During activation of a pentameric ligand-gated ion channel (pLGIC), the binding of agonists promotes the opening of a selective ion conduction pore at a distance of more than 50 Å away from the binding sites. Each subunit consists of a predominantly β-stranded extracellular domain and an α-helical transmembrane pore, which interact via an extended interface. Whereas ELIC forms a cation-selective channel with high conductance that is activated with high efficacy by the primary amines cysteamine, propylamine, and GABA, the cation-selective GLIC is activated by protons and inhibited by bulky positively charged compounds that also act as open channel blockers of the nAChR. Our study has identified a cluster of interacting residues located at the β1-β2 turn, the β6-β7 loop and the pre-M1 region of the extracellular domain, and the M2-M3 loop of the pore that exert a strong influence on channel function.

When mutating Thr28 in ELIC to aspartate, thereby introducing a negative charge that is present in many family members, the EC50 of channel activation shifts to a 45 times lower agonist concentration (18 μM). A similar increase in the affinity was observed in ITC experiments, where the agonist binds with a Keff of 90 μM, a 90-fold decrease in concentration compared to WT, while the binding of the antagonist acetylcholine was unchanged. Patch clamp recordings already show considerable basal activity of this mutant in the absence of ligand and increased currents upon ligand application, whereas no basal activity is observed in WT. The single channel conductance of the mutant is similar to WT, but the current density is lower in both two-electrode voltage clamp and patch clamp experiments. All experiments suggest that this mutant stabilizes a high affinity state with respect to ligand binding, and we were thus interested whether it would be sufficient to change the crystallization behavior and allow us to determine the structure of ELIC in a different conformation. While we succeeded in obtaining crystals of the T28D mutant in the same conditions, they exhibited poorer diffraction than WT and only allowed us to collect data at 4.5 Å in the absence and 9.5 Å in the presence of ligand. The structures indicate that, despite the drastic impact on the potency of the ligand, the mutant crystallized in the familiar nonconducting conformation, which further underlines the stability of this state in a crystalline environment. The role of this interaction in channel activation and the destabilization of the resting state is underlined by a mutation of the respective threonine to aspartate in ELIC, which strongly increases the potency for the agonist and where the channel shows increased basal activity, which is not observed in WT. This basal activity demonstrates that ELIC can, in principle, also open in the absence of agonist and thus underlines the validity of the MWC model also for this channel.

>[10x]APADNAADARPVDVSVSIFINKIYGVNDLEQTYKVDGYIVAQWTGKPRKTPGDKPLIVENTQIERWINNGLWVPALEFINVVGSPDTGNKRLMLFPDGRVIYNARFLGSFSNDMDFRLFPFDRQQFVLELEPFSYNNQQLRFSDIQVYTENIDNEEIDEWWIRGKASTHISDIRYDHLSSVQPNQNEFSRITVRIDAVRNPSYYLWSFILPLGLIIAASWSVFWLESFSERLQTSFTLMLTVVAYAFYTSNILPRLPYTTVIDQMIIAGYGSIFAAILLIIFAHHRQANGVEDDLLIQRCRLAFPLGFLAIGCVLVIRGITL> VMKQYLSRLASLTLFVGFMSAAQAAVAPLDLVQPISDYKI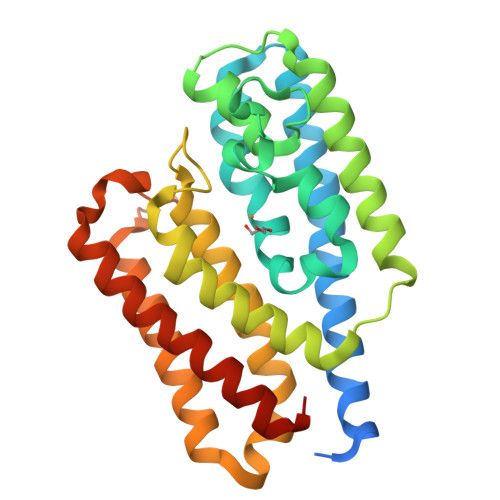YVSENLQTLVRDTREFTNAVKAGDVAKAKKLFASTRMSYERIEPIAELFSDLDASIDSRADDHEKAEKDPAFFGFHRIEYGLFAQNSAKGLAPVADKLMADVLELQKRIRGLTFPPEKVVGGAAVLMEEVAATKISGEEDRYSHTDLWDFQANFEGAKKIVDLFRPLVVKDNRAFADKVDANFDTVFKTLAKYRTADGGFELYGKLSERDRKVLAGRVNTLAEDLSKMRGLLGLDLEHHHHHH>[2x]SGSGSSPELDELWKRVKKLVTELLEQAERAGDPEEIFKLLEVAAALVFLAEMFLRLAAIQEKATDPEIQELAERVLRLIKRLLEEAERAGDPRRIRELVEVA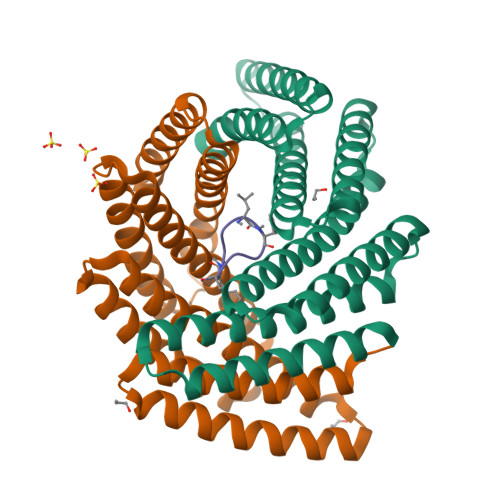SQLAFLLELFYRLKEIQERATDPEIQELAERVLRLIKKLLKAAEEAGDPRKIHKLVFVAIVLLFLLQTFYRLKEIQEKATDPEIQRKAQEVLEKIKRLLEAAERAGDPAKILLYVIRALLLAMELKFAYRKR;> APLFAPLF>MKISG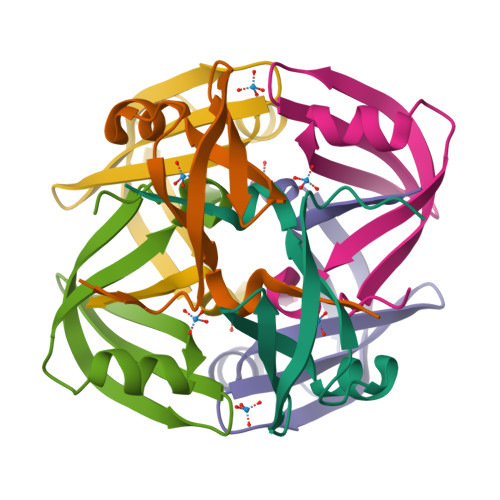RNKLEATVKEIVKGTVMAKIVMDYKGTELVAAITIDSVADLDLVPGDKVTALVKATEMEVLK[12x]> AMKNLFLTSSFKDVVPLFTEFESNLQGKTVTFIPTASTVEEVTFYVEAGKKALESLGLLVEELDIATESLGEITTKLRKNDFIYVTGGNTFFLLQELKRTGADKLILEEIAAGKLYIGESAGAVITSPNIAYI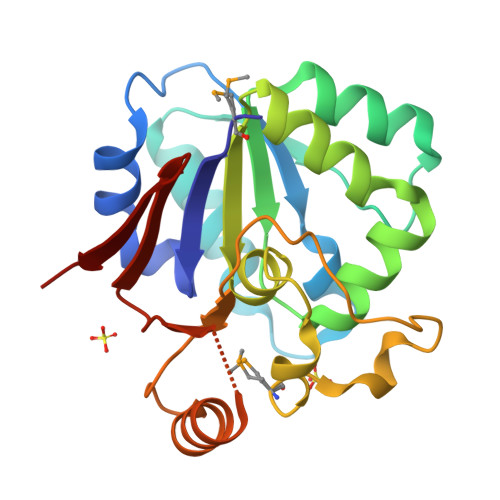QTMDSTKKAVNLTNYDALNLVDFSTLPHYNNTPFKEITQKIVTEYAGKSQIYPISNHEAIFIRGKEVITKRLS> SGISQTVIVGPWGA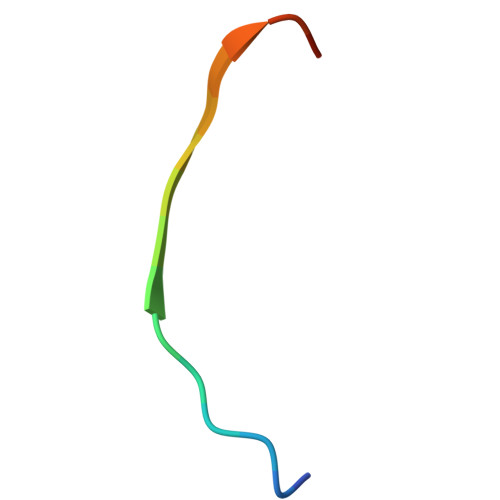KSA>[4x]SNAMTARYIAIDWGSTNLRAWLYQGEECLESRQSEAGVTRLNGRSPAAVLAEITQHWRDGATPVVMAGMVGSNVGWKIAPYLPLPAAFSDIGQQLTAVGDNIWIIPGLCVSRDDNHNVMRGEETQLLGARALAPSSVYVMPGTHCKWVLADRRQIHDFRTVLTGELHHLLLQLSLVGAGLPPQETSAAAFAAGLQRGINNPAVLPQLFE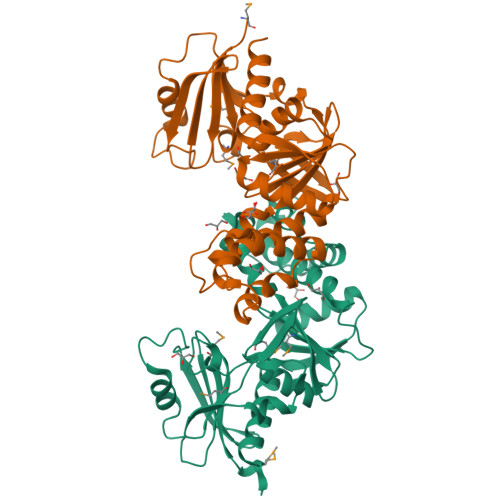VRASHVLGALPREQVSEFLSGLLIGAEVATLSDTFAGQQAISLVAGSSLTSRYQQAFAAIGREVSAVAGDTAFQTGIRSIAYAVAN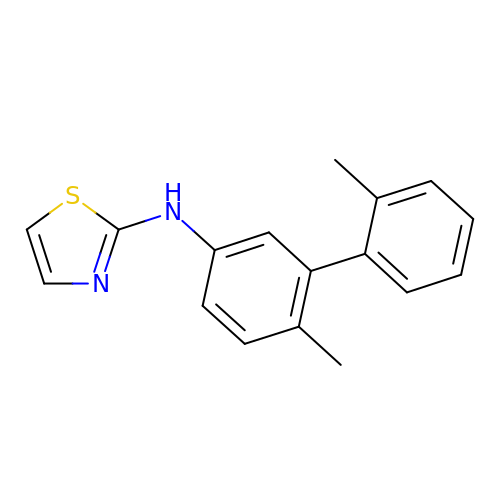N-(2',6-dimethyl[1,1'-biphenyl]-3-yl)-1,3-thiazol-2-amine | C17 H16 N2 S | OZBQQKIXAODXQL-UHFFFAOYSA-N> MSTPARRRLMRDFKRMKEDAPPGVSASPLPDNVMVWNAMIIGPADTPYEDGTFRLLLEFDEEY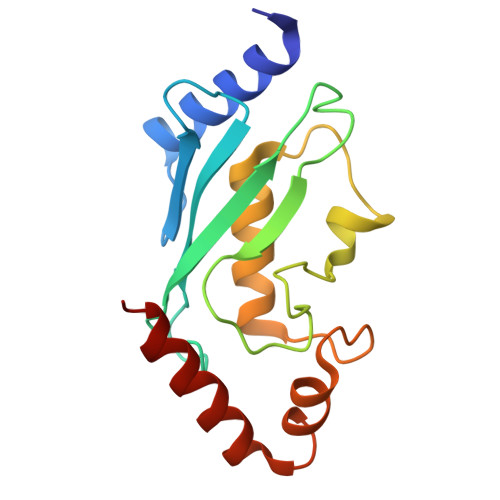PNKPPHVKFLSEMFHPNVYANGEICLDILQNRWTPTYDVASILTSIQSLFNDPNPASPANVEAATLFKDHKSQYVKRVKETVEKSWE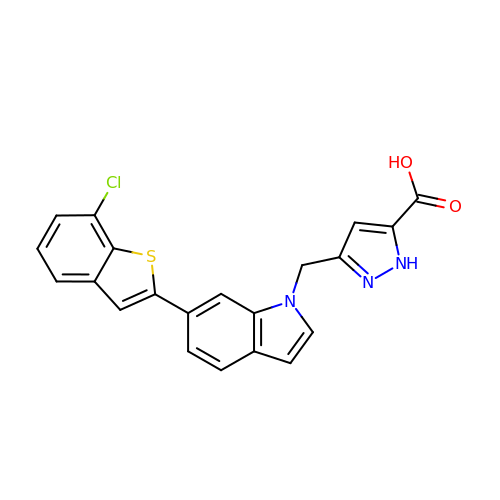3-{[6-(7-chloro-1-benzothiophen-2-yl)-1H-indol-1-yl]methyl}-1H-pyrazole-5-carboxylic acid | C21 H14 Cl N3 O2 S | YGJVVGJDTMKYJP-UHFFFAOYSA-N>[2x]ETGGFPEDSEPISISHGNYTKQYPVFVGHKPGRNTTQRHRLDIQMIMIMNRTLYVAARDHIYTVDIDTSHTEEIYCSKKLTWKSRQADVDTCRMKGKHK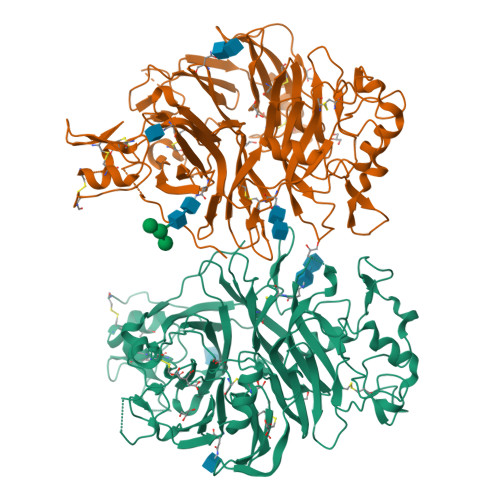DECHNFIKVLLKKNDDTLFVCGTNAFNPSCRNYRVDTLETFGDEFSGMARCPYDAKHANIALFADGKLYSATVTDFLAIDAVIYRSLGDSPTLRTVKHDSKWLKEPYFVQAVDYGDYIYFFFREIAVEYNTMGKVVFPRVAQVCKNDMGGSQRVLEKQWTSFLKARLNCSVPGDSHFYFNILQAVTDVIRINGRDVVLATFSTPYNSIPGSAVCAYDMLDIANVFTGRFKEQKSPDSTWTPVPDERVPKPRPGCCAGSSSLEKYATSNEFPDDTLNFIKTHPLMDEAVPSIINRPWFLRTMVRYRLTKIAVDNAAGPYQNHTVVFLGSEKGIILKFLARIGSSGFLNGSLFLEEMNVYNPEKCSYDGVEDKRIMGMQLDRASGSLYVAFSTCVIKVPLGRCERHGKCKKTCIASRDPYCGWVRESGSCAHLSPLSRLTFEQDIERGNTDGLGDCHNSGTKHHHHHH> GSHMMAQEQTKRGGGGGDDDDIAGSTAAGQERREKLTEETDDLLDEIDDVLEEN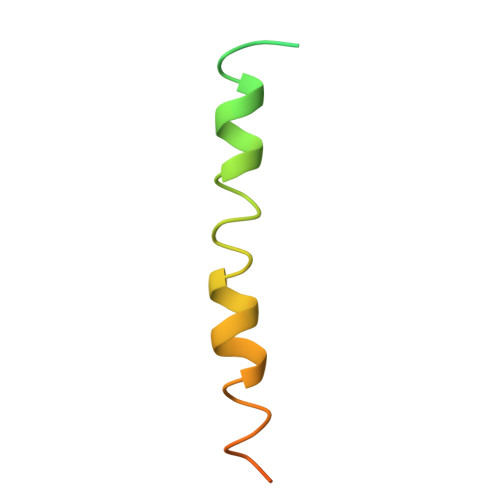AEDFVRAYVQKGGE> VLDLDLFRVDKGGDPALIRETQEKRFKDPGLVDQLVKADSEWRRCRFRADNLNKLKNLCSKTIGEKMKKKEPVGDDESVPENVLSFDDLTADALANLKVSQIKKVRLLIDEAILKCDAERIKLEAE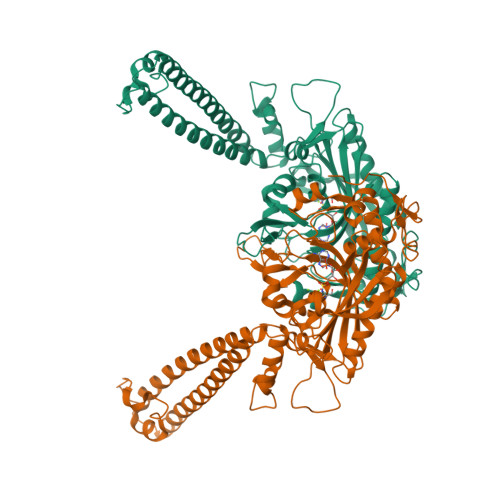RFENLREIGNLLHPSVPISNDEDVDNKVERIWGDCTVRKKYSHVDLVVMVDGFEGEKGAVVAGSRGYFLKGVLVFLEQALIQYALRTLGSRGYIPIYTPFFMRKEVMQEVAQLSQFDEELYKVIGKGSEKSDDNSYDEKYLIATSEQPIAALHRDEWLRPEDLPIKYAGLSTCFRQEVGSHGRDTRGIFRVHQFEKIEQFVYSSPHDNKSWEMFEEMITTAEEFYQSLGIPYHIVNIVSGSLNHAASKKLDLEAWFPGSGAFRELVSCSNCTDYQARRLRIRYGQTKKMMDKVEFVHMLNATMCATTRTICAILENYQTEKGITVPEKLKEFMPPGLQELIPFVKPAPIE>MKMYEVKEFSSGKRKLEDYKSIIGEEEVSKIQEKAEKLKGRSFVHVNSTSFGGGVAEILHSLVPLLRSIGIEARWFVIEGPTEFFNVTKTFHNALQGNESLKLTEEMKELYLNVNRENSKFIDLSSFDYVLVHDPQPAALIEFYEKKSPWLWRCHIDLSSPNREFWEFLRRFVEKYDRYIFHLPEYVQPELDRNKAVIMPPSIDPLSEKNVELKQTEILRILERFDVDPEKPIITQVSRFDPWKGIFDVIEIYRKVKEKIPGVQLLLVGVMAHDDPEGWIYFEKTLRKIGEDYDVKVLTNLIGVHAREVNAFQRASDVILQMSIRAGFGLTVTEAMWKGKPVIGRAVGGIKFQIVDGETGFLVRDANEAVEVVLYLLKHPEVSKEMGAKAKE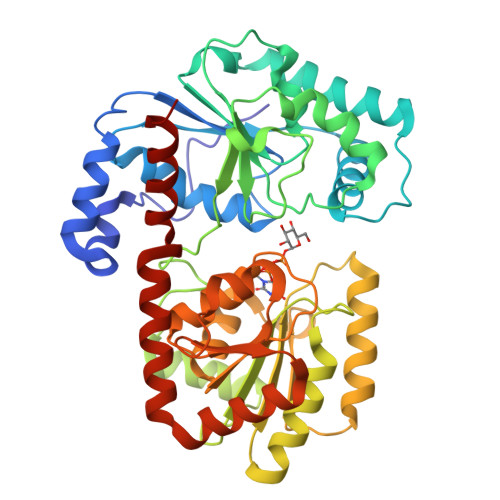RVRKNFIITKHMERYLDILNSLGG[2x]> SNAMTISEARLSPQVNLLPIKRHSNEEVEETAAILKKRTIDNEKCKDSDPGFGSLQRRLLQQLYGTLPTDEKIIFTYLQDCQQEIDRIIKQSIIQKESHSVILVGPRQSYKTYLLDYELSLLQQSYKEQFITIRLNGFIHSEQTAINGIATQLEQQLQKIHGSEEKIDDTSLETISSGSLTEVFEKILLLLDSTTKTRNEDSGEVDRESITKITVVFIFD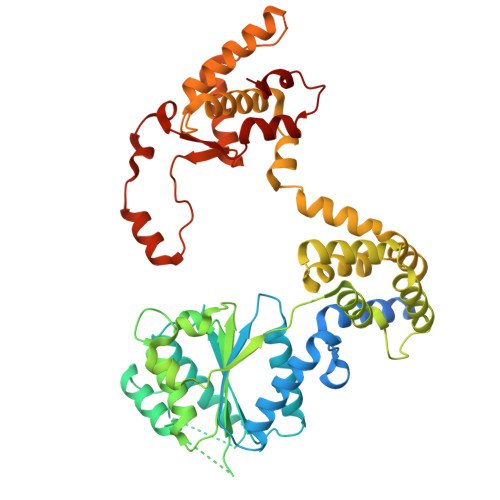EIDTFAGPVRQTLLYNLFDMVEHSRVPVCIFGCTTKLNILEYLEKRVKSRFSQRVIYMPQIQNLDDMVDAVRNLLTVRSEISPWVSQWNETLEKELSDPRSNLNRHIRMNFETFRSLPTLKNSIIPLVATSKNFGSLCTAIKSCSFLDIYNKNQLSNNLTGRLQSLSDLELAILISAARVALRAKDGSFNFNLAYAEYEKMIKAINSRIPTVAPTTNVGTGQSTFSIDNTIKLWLKKDVKNVWENLVQLDFFTEKSAVGLRDNATAAFYASNYQFQGTMIPFDLRSYQMQIILQELRRIIPKSNMYYSWTQL> MTKQEKTALNMARFIRSQTLTLLEKLNELDPD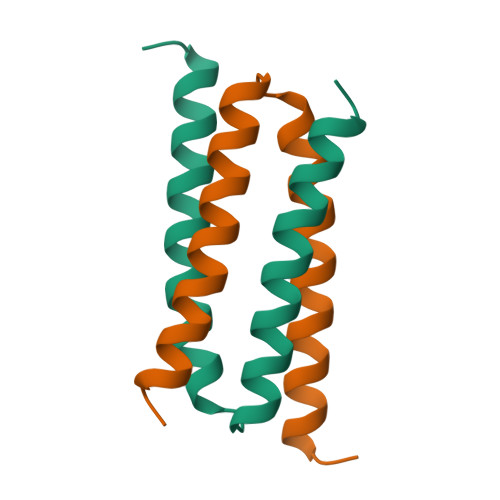EQADICESLHDHADELYRSCLARFGDDGENL>GGGRDEHPDARRQAQLRHLLLQDCGSCHGLRLTGGLGPALTPEALRGKPRESLVATVLMGRPQTPMPPWAGLLSADDA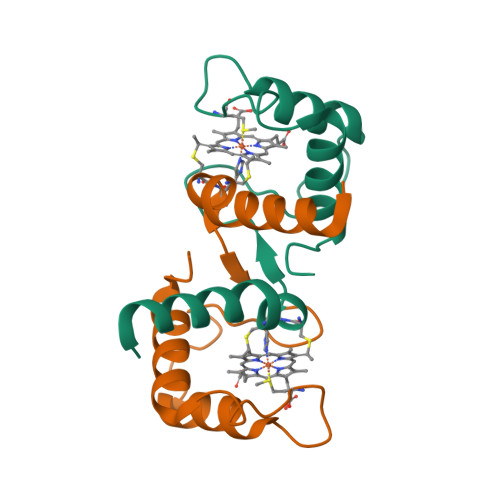GWLVDRLIEGEIAP[11x]> MENTENSVDSKSIKNLEPKIIHGSESMDSGISLDNSYKMDYPEMGL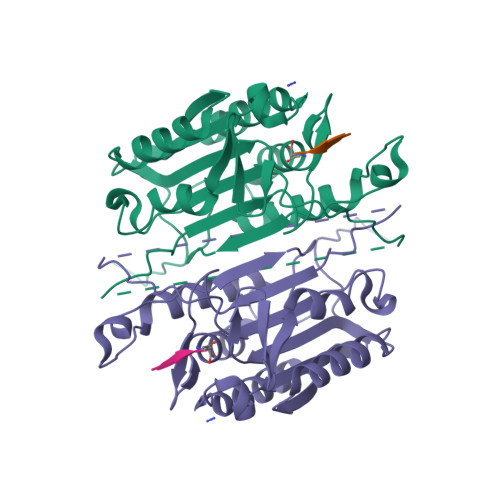CIIINNKNFHKSTGMTSRSGTDVDAANLRETFRNLKYEVRNKNDLTREEIVELMRDVSKEDHSKRSSFVCVLLSHGEEGIIFGTNGPVDLKKITNFFRGDRCRSLTGKPKLFIIQACRGTELDCGIETDSGVDDDMACHKIPVEADFLAAYSTAPGYYSWRNSKDGSWFIQSLCAMLKQYADKLEFMHILTRVNRKVATEFESFSFDATFHAKKQIPCIHSMLTKELYFYHH>[2x]NNNGACU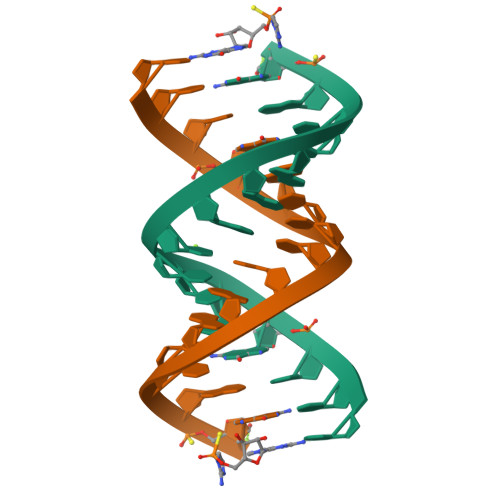UAAGUCGG>[3x]MYSIEVRTHSA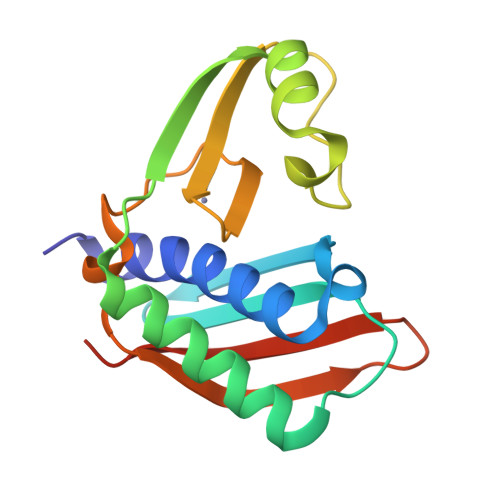LHVVKGAVVKVLGSEAKWTYSTYVKGNKGVLIVKFDRKPSDEEIREIERLANEKVKENAPIKIYELPREEAEKMFGEDMYDLFPVPEDVRILKVVVIEDWNVNACNKEHTKTTGEIGPIKIRKVRFRKSKGLLEIHFELLELENPS>[2x]MQTTVTTMLLASVALAACAGGGSTPLPLPQQQPPQQEPPPPPVPLASRAACEALKDGNGDMVWPNAATVVEVAAWRDAAPATASAAALPEHCEVSGAIAKRTGIDGYPYEIKFRLRMPAEWNGRFFMEGGSGTNGSLSAATGSIGGGQIASALSRNFATIATDGGHDNAVNDNPDALGTVAFGLDPQARLDMGYNSYDQVTQAGKAAVARFYGRAADKSYFIGCSEGGREGMMLSQRFPSHYDGIVAGAPGYQLPKAGISGAWTTQSLAPAAVGLDAQGVPLI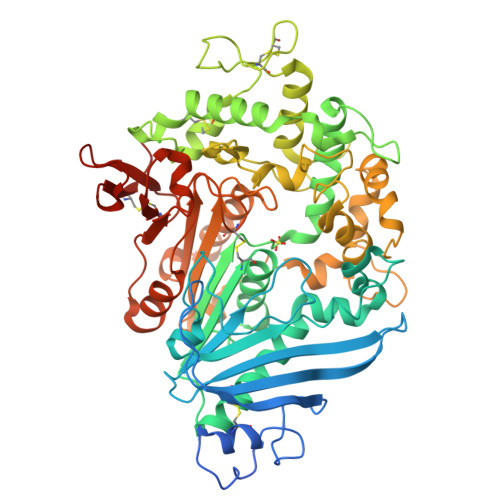NKSFSDADLHLLSQAILGTCDALDGLADGIVDNYRACQAAFDPATAANPANGQALQCVGAKTADCLSPVQVTAIKRAMAGPVNSAGTPLYNRWAWDAGMSGLSGTTYNQGWRSWWLGSFNSSANNAQRVSGFSARSWLVDFATPPEPMPMTQVAARMMKFDFDIDPLKIWATSGQFTQSSMDWHGATSTDLAAFRDRGGKMILYHGMSDAAFSALDTADYYERLGAAMPGAAGFARLFLVPGMNHCSGGPGTDRFDMLTPLVAWVERGEAPDQISAWSGTPGYFGVAARTRPLCPYPQIARYKGSGDINTEANFACAAPPLEHHHHHH> MEYNFQALAELYKNALLNDVLSFWEKYSLDWQQGGYFTCLDREGKIYDTDKFIWLQNRQVWTFSMLYNQLEKRENWLKIASNGANFLAQHGRDSDGNWYFALTREGKPLVHPYNIFSDCFAAMAFSKYALAGGEEWAKDVAMQAYNNVLRRKDNPKGKYNKTYPGTRPMKSLAVPMILANLTLEMEWLLPKETLENVLAETVREVMTDFLDQERGLMYENVAPDGSHIDCFEGRLINPGHGIEAMWFIMDIARRQNDTKTINQAVDVVLNILNFAWDSEYGGLYYFMDADGHPPQQLEWDQKLWWVHLESLVALAMGYRLTGREACWEWYQKMHDYAWSHFADSEYGEWFGYLNRRGEVLLNLKGGKWKGCFHVPRALYLCWQQFEAIATPLQHHHHHH

N-Acetylglucosamine 2-epimerases (AGEs; EC 5.1.3.8) catalyze the reversible epimerization of N-acetylmannosamine (ManNAc) to N-acetylglucosamine (GlcNAc) in both eukary­otic and prokaryotic cells. The reaction follows a deprotonation/reprotonation mechanism involving two key residues, which had been thought to be histidines, but which have recently been identified as a glutamine and an arginine. AGE activity is greatly enhanced by the presence of nucleotides, in particular ATP, which serve as allosteric activators.

In this study, we report the determination of the crystal structure of the AGE from the local strain Nostoc sp. KVJ10, which we refer to as nAGE10. In contrast to the pAGE and AnaAGE crystals, which both belonged to space group P212121, the nAGE10 crystal belonged to space group P42212. The structure of the monomer was resolved for the amino-acid sequence from Tyr3 to Leu391, with residues 157–164 missing. The fold is that of an (α/α)6 barrel, with the helices connected by small loops at one end (the back) and long loops at the other end (the front). Gel filtration showed that nAGE10 was present as a dimer, and a melting temperature of 72.3°C was determined by DSC. The nAGE10 dimer, which involves the front faces of each monomer, differs from the back-to-back association presented for AnaAGE and pAGE. A comparison of the assembly parameters calculated by the PISA method indicates that the front-to-front organization is more favourable than the back-to-back organization in terms of interface area, number of interactions and solvation energy. One of the principal consequences of the front-to-front dimer is for the ATP-binding site. Independently of which site is used, the localization of the ATP-binding site at the dimer interface is the determinant of its role in AGE activity, which may involve the oligomeric state of the enzyme.>MGTPKPRILPWLVSQLDLGQLEGVAWVNKSRTRFRIPWKHGLRQDAQQEDFGIFQAWAEATGAYVPGRDKPDLPTWKRNFRSAL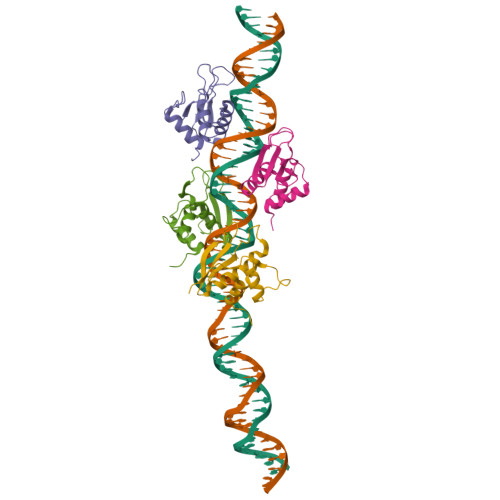NRKEGLRLAEDRSKDPHDPHKIYEFVNSGVGDFSQPDTS[4x]> MLAKNKGKIPGLKIDQKIRGQMPERGWTEDDIKNTVSNGATGTSFDKRSPKKTPPDYLGRNDPATVYGSPGKYVVVNDRTGEVTQ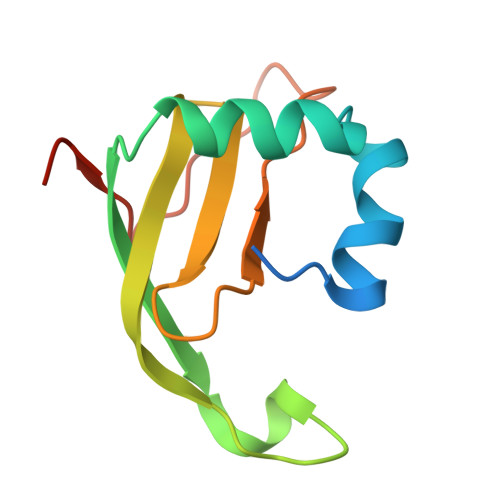ISDKTDPGWVDDSRIQWGNKNDQ AK is a small enzyme that catalyzes a reversible phosphoryl transfer reaction between ATP/AMP and two ADPs. The structures comprised the characteristic three-domain arrangement: the CORE (residues 1–38, 69–136, and 143–193), AMPbind (residues 39–68), and LID (residues 137–142) domains. The static CORE domain provides substrate-binding sites, and the dynamic AMPbind and LID domains close over the AMP and ATP sites, respectively, upon substrate binding. AK is a small protein that undergoes relatively large conformational changes upon substrate binding and product release, and has long been used as a model system for studying connections between structure, function, and dynamics.

In this study, we solved the crystal structure of AK1 from the Antarctic fish Notothenia coriiceps (AKNc), and characterized its thermal stability and temperature–activity profile. To assess the structural basis of cold adaptation, we determined the crystal structures of AKNc and AKDr to resolutions of 1.99 and 1.75 Å, respectively, using molecular replacement. The Tm of AKNc was significantly lower than those of homologues from tropical fishes, indicating the thermal stability of AKNc is substantially reduced compared with those of the other three AKs. In the structure of AKNc, Val28 in the N-terminal α1 helix interacts closely (<4 Å) with conserved hydrophobic residues in the β3 strand (Leu91) and the C-terminal α9 helix (Phe183, Val186, and Ile190). In the CORE domain of AKNc, we found two additional Val residues (Val118 and Val173), around which hydrophobic packing could be improved by mutations. Val118 and Val173 of AKNc are adjacent to each other (<4 Å) in β4 and β5, respectively. Their side chains are found in the hydrophobic interior of the CORE domain, making contacts with residues in β1, α1, and α9 such as Val13, Lys21, Val182, and Val186. However, there is room for improvement in hydrophobic packing around the two Val residues (Val118 and Val173). Taken together, the structural analyses of AKNc and AKDr suggest that hydrophobic CORE packing is not optimal in AKNc, and is important in thermal stability of fish AKs. In the present study, we discovered suboptimal hydrophobic packing in the CORE domain of the Antarctic fish AK.

>GHMADKIKDAKIIFVVGGPGSGKGTQCEKVVAKYGYTHLSSGDLLRAEVSSGSERGKQLQAIMQKGELVPLDTVLDMIKDAMIAKADVSKGYLIDGYPREVKQGEEFEKKIGKPCLLLYVDAKGETMVKRLMKRGETSGRADDNEETIKKRLDLYYKATEPVIAFYEGRGIVRKVDSELPVDEVFKQVSTAIDAL[2x]> MLTPTRRLPKALSPYAQA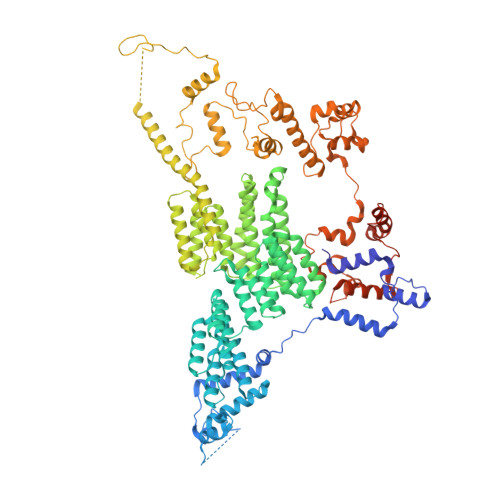LRHVALRGATAFGPGAKEMELDMLRKGTLPADYRPPVQGRWDDTIERWAYAWQFPAEEEQDDITKSVERNASGMQALLEIGNKLLRSPPSPEPLSGKASKLYPPVGDMSSGNTALLPPNPTYDVLEQDVSELMAEDAVVVTSQPRLRAEELSAKYNVPMAYIDDSSEASNASKSLALVMEDVGLEFTEDGLTVVISALSRQGYGTIGRAIFDFASAMGLGPSAEMYRALMKYASRRGDVNESMALIEEMKGNGITPRIGNWHELMYTFYKAKDYPAVSQIVDNMKMYANIEPNEVTFVLQLKALAKDNSQLNSLPEAIQLFDQMENVYGFIASRPHYDAMMFHLSQSPRPEMRLRCEELAHKMELMGIVWNANTYLNLIRSAQVVGDVAAVEKYLSRMREEGIPASIGHLTWAVQAHVQSMIRIDYDALKEKDESPLPTWLEHLETCFGIYELVVRRGWVMQLPFVNALLRLTCQATILSMERTPDEAETIGRFEEQANKIWNHTFDEWQLQKDVYSYECYIALLAHQQRIDEAEKLFQEMILKKDLSPSRRTYHCMIFMHLSSGEEGGTARALRYLEAMERAGIQVRPSLLKKIVRVNNAAGYKRDMKRRARRIMQAREEYLARKEEGVSFGEGGKEGASNQRADVDAEGNSILEPLAVSPTSTLAWWEKWKRETVSKHELFTEEGADGTPKGETFEEKNEALRMMGITSSFQTKDLVPQPDRQKLLPLIRREEGEIAGSLWAMDGGELSYPKDGGGPQGWGVRLWRERQLVKREYQKVLDGYRPVPQLSTLGNSVRTAGDQLDIERSGAQTPGELSDYRNFPDNRFDGGQLKPESEAAPAVPFSAELVWQGEANDKLSPYKSDEEIALENDNTFFSSLSKETEGKLSIAVKAMQNKEENSVDVRGKGVTRRSKFDYLEKWRDMYRHGTLEVPEGPTLNFGRTPDDHKETMAALVRGWYQRNRKEPASEEELKRWRVDEQRSSETSASRAALKKRKQVRSRHRNK> GTAKGHNPTEFPTIYDASSAPTAANTTVGIITIGGVSQTLQDLQQFTSANGLASVNTQTIQTGSSNGDYSDDQQGQGEWDLDSQSIVGSAGGAVQQLLFYMADQSASGNTGLTQAFNQAVSDNVAKVINVSLGWCEADANADGTLQAEDRIFATAAAQGQTFSVSSGDEGVYECNNRGYPDGSTYSVSWPASSPNVIAVGGTTLYTTS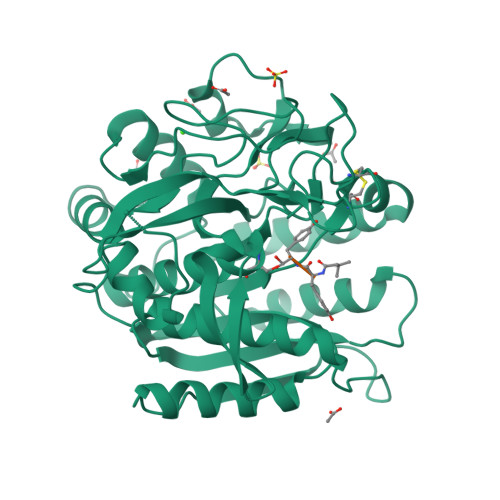AGAYSNETVWNEGLDSNGKLWATGGGYSVYESKPSWQSVVSGTPGRRLLPDISFDAAQGTGALIYNYGQLQQIGGTSLASPIFVGLWARLQSANSNSLGFPAASFYSAISSTPSLVHDVKSGNNGYGGYGYNAGTGWDYPTGWGSLDIAKLSAYIRSNGF2-[8-azanyl-2-(2-fluoranylpyridin-4-yl)-1,7-naphthyridin-5-yl]propan-2-ol | C16 H15 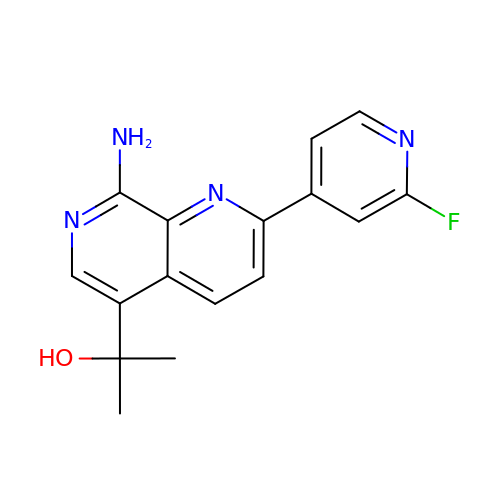F N4 O | XVUSMHCLFMFBQR-UHFFFAOYSA-N>[2x]LADSSDVTEVE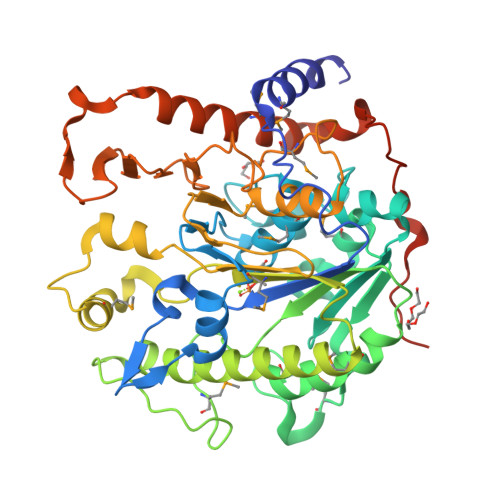NYMKANYDVPNNVYFGKAEGKNVIYVSLESLQSFIIDYKIDGKEVTPFLNKLAHDNETFYFDNFFHQTGQGKTSDAEFMMENSLYPLAQGSVFVNKAQNTLQSVPAILKSKNYTSATFHGNTQTFWNRNEMYKAEGIDKFFDSAYYDMNEENTKNYGMKDKPFFKESMPLLESLPQPFYTKFITLSNHFPFGMDEGDTDFPAGDFGDSVVDNYFQSAHYLDQSIEQFFNDLKKDGLYDKSIIVMYGDHYGISENHNKAMAKVLGKDEITDYDNAQLQRVPLFIHAAGVKGEKVHKYAGDVDVAPTILHLLGVDTKDYLMSGSDILSKEHREVIPFRNGDFISPKYTKISGKYYDTKTGKELDESEVDKSEDSLVKKELEMSDKIINGDLLRFYEPKGFKKVNPSDYDYTKHDEDSSETSKDNEDK> MGSSHHHHHHSSPISPIETVPVKLKPGMDGPKVKQWPLTEEKIKALVEICTEMEKEGKISKIGPENPYNTPVFAIKKKDSTKWRKLVDFRELNKRTQDFWEVQLGIPHPAGLKKKKSVTVLDVGDAYFSVPLDEDFRKYTAFTIPSINNETPGIRYQYNVLPQGWKGSPAIFQSSMTKILEPFRKQNPDIVIYQYVDDLYVGSDLEIGQHRTKIEELRQHLLRWGLTTPDKKHQKEPPFLWMGYELHPDKWTVQPIVLPEKDSWTVNDICKLVGKLNWASQIYPGIKVRQLSKLLRGTKALTEVIPLTEEAELELAENREILKEPVHGVYYDPSKDLIAEIQKQ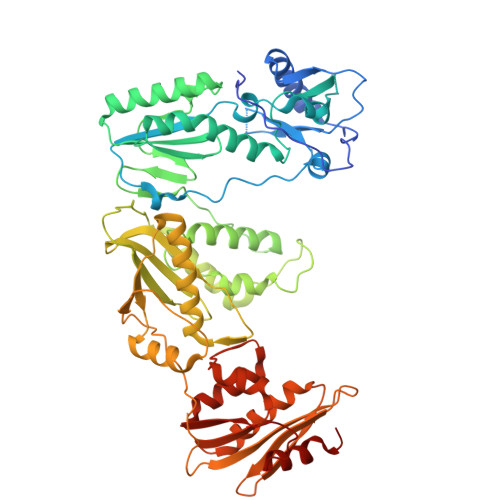GQGQWTYQIYQEPFKNLKTGKYARMRGAHTNDVKQLTEAVQKITTESIVIWGKTPKFKLPIQKETWETWWTEYWQATWIPEWEFVNTPPLVKLWYQLEKEPIVGAETFYVDGAANRETKLGKAGYVTNRGRQKVVTLTDTTNQKTELQAIYLALQDSGLEVNIVTDSQYALGIIQAQPDQSESELVNQIIEQLIKKEKVYLAWVPAHKGIGGNEQVDKLVSAGIRKVL1-[4-(cyanomethyl)-1-[(4-phenylphenyl)methyl]piperidin-4-yl]-3-(cyclopropylcarbonylamino)pyrazole-4-carboxamide 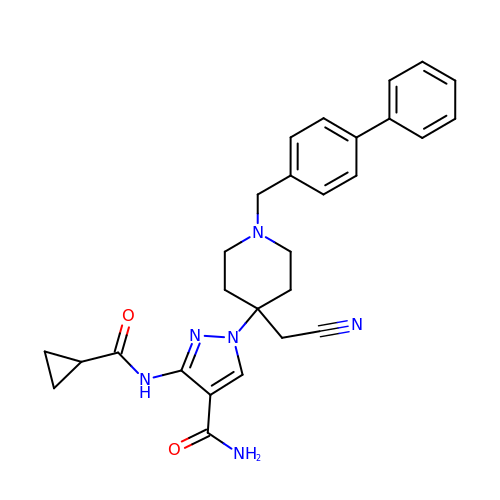| C28 H30 N6 O2 | HKYCPTFBXARDTR-UHFFFAOYSA-N> GHMSAHVQQDKYETNVSYKKLNQLAPYFKGFDGSFVLYNEREQAYSIYNEPESKQRYSPNSTYKIYLALMAFDQNLLSLNHTEQQWDKHQYPFKEWNQDQNLNSSMKYSVNWYYENLNKHLRQDEVKSYLDLIEYGNEEISGNEN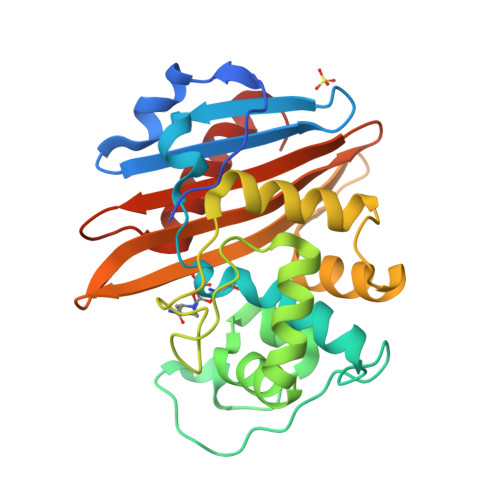YWNESSLKISAIEQVNLLKNMKQHNMHFDNKAIEKVENSMTLKQKDTYKYVGKTGTGIVNHKEANGWFVGYVETKDNTYYFATHLKGEDNANGEKAQQISERILKEMELI>MHHHHHHSSGRENLYFQGPEQPFIVLGQEEYGEHHSSIMHCRVDCSGRRVASLDVDGVIKVWSFNPIMQTKASSISKSPLLSLEWATKRDRLLLLGSGVGTVRLYDTEAKKNLCEININDNMPRILSLACSPNGASFVCSAAAPSLTSQVDFSAPDIGSKGMNQVPGRLLLWDTKTMKQQLQFSLDPEPIAINCTAFNHNGNLLVTGAADGVIRLFDMQQHECAMSWRAHYGEVYSVEFSYDENTVYSIGEDGKFIQWNIHKSGLKVSEYSLPSDATGPFVLSGYSGYKQVQVPRGRLFAFDSEGNYMLTC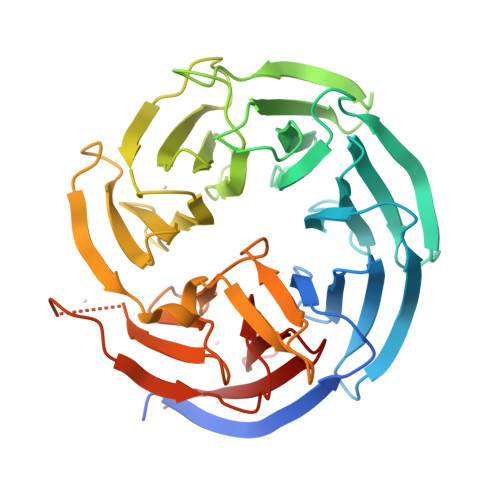SATGGVIYKLGGDEKVLESCLSLGGHRAPVVTVDWSTAMDCGTCLTASMDGKIKLTTLLAHKA[2x]>[5x]EKNVSIVVAASVLSSGIGINGQLPWSISEDLKFFSKITNNKCDSNKKNALIMGRKTWDSIGRRPLKNRIIVVISSSLPQDEADPNVVVFRNLEDSIENLMNDDSIENIFVCGGESIYRDALKDNFVDRIYLTRVALEDIEFDTYFPEIPETFLPVYMSQTFCTKNISYDFMIFEKQEKKTLQNCDPARGQLKSIDDTVDLLGEIFGIRKMGNRHKFPKEEIYNTPSIRFGREHYEFQYLDLLSRVLENGAYRENRTGISTYSIFGQMMRFDMRESFPLLTTKKVAIRGIFEELIWFIKGDTNGNHLIEKKVYIWSGNGSKEYLERIGLGHREENDLGPIYGFQWRHYNGEYKTMHDDYTGVGVDQLAKLIETLKNNPKDRRHILTAWNPSALSQMALPPCHVLSQYYVTNDNCLSCNLYQRSCDLGLGSP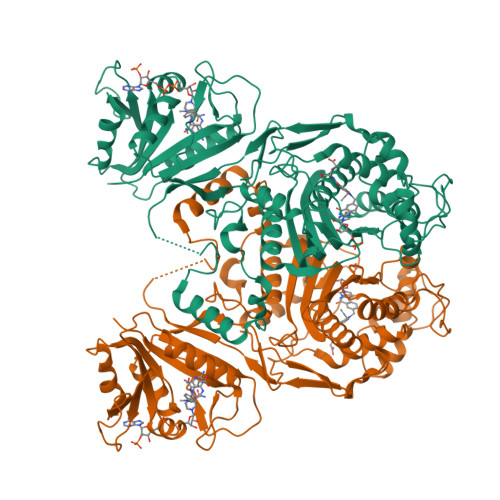FNIASYAILTMMLAQVCGYEPGELAIFIGDAHIYENHLTQLKEQLSRTPRPFPQLKFKRKVENIEDFKWEDIELIGYYPYPTIKMDMAV>HHHHHHMTDRFTRLLGIQQPIIQAPMLGVSTPALAAAVSNAGGLGSIAITGSAAEKGRALIREVRGLTDKPFNVNLFCHRPGQADPARERAWLDYLKPLFAEFGAEPPVRLKNIYLSFLEDPTLLPMLLEERPAAVSFHFGAPPRDQVRALQAVGIRVLVCATTPEEAALVEAAGADAVVAQGIEAGGSRGVFEPERGDAAIGTLALVRLLAARGSLPVVAAGGIMDGRGIRAALELGASAVQMGTAFVLCPESSANAAYREALKGPRAARTALTVTMSGRSARGLPNRMFFDAA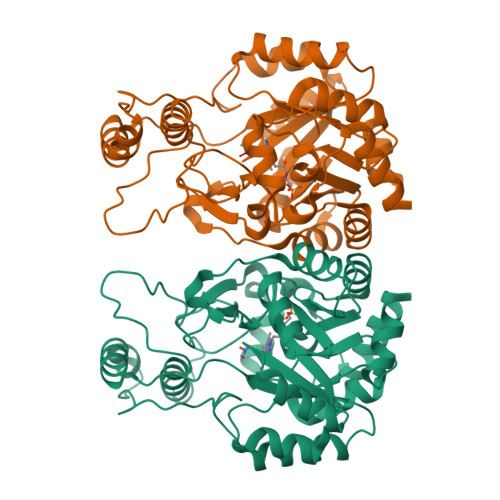APGVPPLPDYPFVYDATKALQTAALARGNHDFAAQWAGQGAALARELPAAELLRTLVEELRG[2x]> SAEQVEKLRNKINNAAVLVFAKSFCPYCKKVMERFNNLKIPFGYLDLDLKKNGSDYQKMLQEITGRTTVPQVFFRGEFIGGCDDVMAIDDDTIVKKANEMKYDYDMVIIGGGSGGLALAKESAKSGAKVALLDFVVPTPMGTTWGLGGTCVNVGCIPKKLMHQAALLNHYMEDAKSFGWDVDKGPHDWVKMVEGIQDHIHALNFGYRSSMMNANVKYLNALGEIVDPHTIKTTNKQGIVKNITTNTIIVATGERPRYPPIPGAKEYGITSDDLFTLDHNPGKTLCVGASYVSLECAGFLSSIGCDVTVMVRSIFLRGFDQQMAGLISDYIAKYGVKFVRPCVPTSVRCLEEYDPESGKLAIYEVEGKHEDGTPFKDTFNTVLFAVGRDPCTTNIGLQNVDVKTTNGRVVVDDEERTNVPNIYAIGDVSNAGYQLTPLAIQAGKNLARRLYTADDCRTDYTNVPTTVFTPLEYGCIGLSEENAISKFGEDNIEV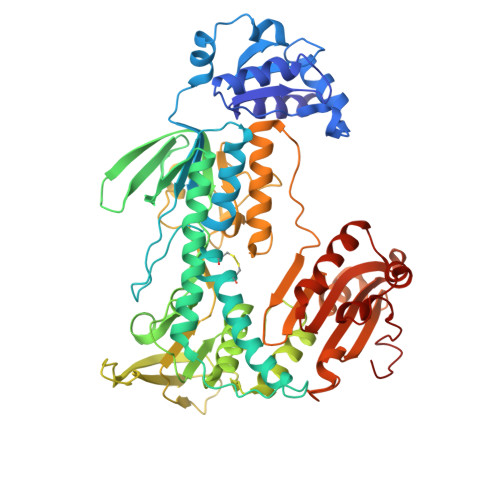FHSYFQPLEWTVPHRPDNTCYAKLIINKQDDNRVVGFHVFGPNAGEVTQGYAVAMHLGARKEDFDRTIGIHPTCSETFTTLRVTKSSGASA> GSPGISGGGGGSHIEGYECQPIFLNVLEAIEPGVVCAGHDNNQPDSFAALLSSLNELGERQLVHVVKWAKALPGFRNLHVDDQMAVIQYSWMGLMVFAMGWRSFTNVNSRMLYFAPDLVFNEYRMHKSRMYSQCVRMRHLSQEFGWLQITPQEFLCMKALLLFSIIPVDGLKNQKFFDELRMNYIKELDRIIACKRKNPTSCSRRFYQLTKLLDSVQPIARELHQFTFDLLIKSHMVSVDFPEMMAEIISVQVPKILSGKVKPIYFHTQ;> SRWQALFDDGTDTSR

The androgen receptor (AR) is the cellular mediator of the actions of the hormone 5-α dihydrotestosterone (DHT). Androgen binding to AR leads to activation of genes involved in the development and maintenance of the male reproductive system and other tissues such as bone and muscle. AR is distinguished from other nuclear receptors in that after hormone binding, it preferentially responds to a specialized set of coactivators bearing aromatic-rich motifs, while responding poorly to coactivators bearing the leucine-rich “NR box” motifs favored by other nuclear receptors. Structures of AR in complex with FxxLF, LxxLL, FxxLW, WxxLF, WxxVW, FxxFF, and FxxYF motifs reveal a changing surface of the AR coactivator binding interface that permits accommodation of both AR-specific aromatic-rich motifs and canonical leucine-rich motifs.

To understand how the AR AF-2 accommodates tryptophan residues, structures of AR in complex with peptides containing tryptophan substitutions at the +1 or +5 position, or both, were determined. Surprisingly, WxxLF, analogous to the only tryptophan-containing motif known in vivo, WHTLF in the AR NTD, was relatively disordered, with the peptide displaying the highest B-factor and least well defined density, suggesting that it binds with the lowest affinity. Nonetheless, each of the tryptophan peptides adopted similar helical conformations. Ser−2 of WxxLF similarly interacts with Glu897, but is too distant for helical-capping interactions with the +2 amide group. Instead, Glu893, in a more typical interaction with the +1 amide nitrogen, caps the WxxLF helix. WxxLF also makes backbone interactions with an alternate charge clamp residue, Glu893, pointing towards adaptability in AR AF-2 charge clamp formation. The benzyl moiety of the indole side chains superimpose with the corresponding benzyl side chains of the phenylalanine-rich motifs, effectively mimicking interactions of a phenylalanine residue. However, the presence of a hydrogen-bonding partner on the indole side chain enables an additional polar interaction not seen in the phenylalanine-rich motifs between the indole nitrogen and Gln738.> GAHMVTSNVVL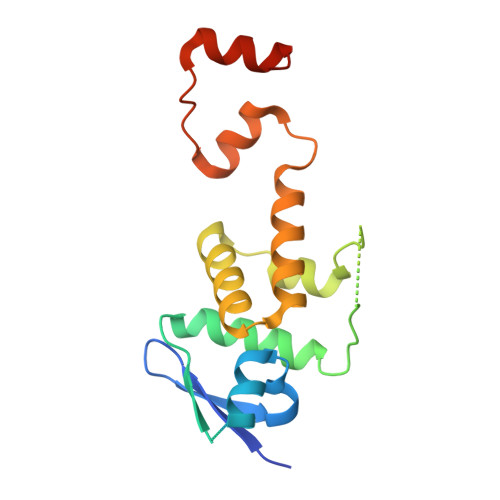VSGEGERFTVDKKIAERSLLLKNYLNDMGDDDDEDDDEIVMPVPNVRSSVLQKVIEWAEHHRDSNFPDEDDDDSRKSAPVDSWDREFLKVDQEMLYEIILAANYLNIKPLLDAGCKVVAEMIRGRSPEEIRRTFNIVNDFTPEEEAAIRRENEWAEDR Herein, we report the first structural and kinetic characterization of a novel alkyl diamine N-hydroxylase DesB from Streptomyces sviceus (SsDesB). This enzyme catalyzes the first committed step in the biosynthesis of desferrioxamine B, a clinical drug used to treat iron overload disorders. Using the electron donor NADPH and molecular oxygen, NMOs catalyze the first committed step in hydroxamate siderophore biosynthesis by oxidizing a primary amine in alkyl amines and amino acids, such as lysine and ornithine, to N-hydroxylated products. SsDesB crystallized as a homotetramer with each protomer consisting of two dinucleotide-binding Rossman-fold domains: an FAD-binding domain (red) and an NADPH-binding domain (blue).

The higher resolution 2.37 Å structure of the ternary complex shows that the NADP+ cofactor is held in the active site pocket in an elongated manner via several direct hydrogen bonds to SsDesB and a network of water-mediated hydrogen bonding bridges between SsDesB residues and NADP+. The electron density is well-defined for both the FAD and NADP+ cofactors, including the nicotinamide ring, in all 8 protomers in the asymmetric unit. The nicotinamide ring is held in position by hydrogen bonding interactions between the nicotinamide N7N atom and main chain carbonyl oxygen atom of H59 and the N5 atom of the FAD isoalloxazine ring. The nicotinamide O7N atom participates in water-mediated hydrogen bonding interactions via water 679 to the E202 side chain and H50 main chain carbonyl oxygen atom. The side chain of Q61 also contributes to stabilizing interactions via a hydrogen bond between the side chain OE1 oxygen atom and the O2D ribose oxygen atom. The phosphate moiety of NADP+ is held in place by a salt bridge between the O2X oxygen and the side chain of K264, and the R232 side chain to the O2X and O1X oxygen atoms. In addition, there is a hydrogen bond between the O3X oxygen and the side chain of S224. There are no significant global structural changes observed upon binding of the NADP+ molecule (r.m.s.d. = 0.26 over 2741 aligned atoms). In comparison to the holoenzyme structure, upon NADP+ binding, several structural adjustments are observed among the residues surrounding the NADP+ binding pocket. At the interface of the FAD isoalloxazine ring and NADP+ nicotinamide ring, the side chain of Q61 shifts away from the FAD isoalloxazine to accommodate the binding of the nicotinamide ring of NADP+, which in turn, induces a shift in the rotamer positions of the nearby L230, E231, and Y232 side chains.

>[8x]MTARPENPSTVHDFVGIGLGPFNLGLACLTEPIDELDGIFLESKPDFEWHAGMFLDGAHLQTPFMSDLVTLADPTSPYSFLNYLKEKGRLYSFYIRENFYPLRVEYDDYCRWAANKLSSIRFGTTVTEVRYEDDLYVVTTSAGDVYRARHLVLGTGTPPYIPEACQGLDGDFIHNSRYVQHRSELVKKESITIVGSGQSAAEIYQDLLGEIDVHGYRLNWVTRSPRFFPLEYTKLTLEMTSPEYIDYYRELPEATRYRLTAEQKGLFKGIDGDLINEIFDLLYQKNLAGPVPTRLLTNSSLNSARHENGTYTLAFRQEEQGKDFEIESQGLVLATGYKYAEPEFLAPVKDRLVYDSQGNFDVSRAYAIDVTGRGVFLQNAGVHTHSITSPDLGMGAYRNSCIIRELLGTEYYPVEKTIAFQEFSV> HRRVKVLLYGQVVGELSQNDSGFLFQYAHDYHGPAISISLPVAQRQFPSETLHPYFASLAPEGWLRQRYSQIQHRDENDLLGM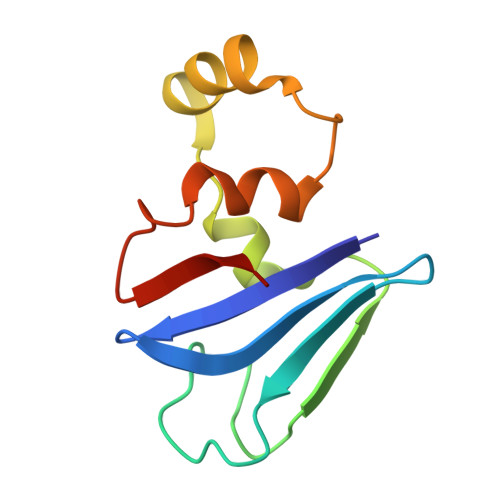LIDNGKNLLGAIQILPWEE>[15x]SM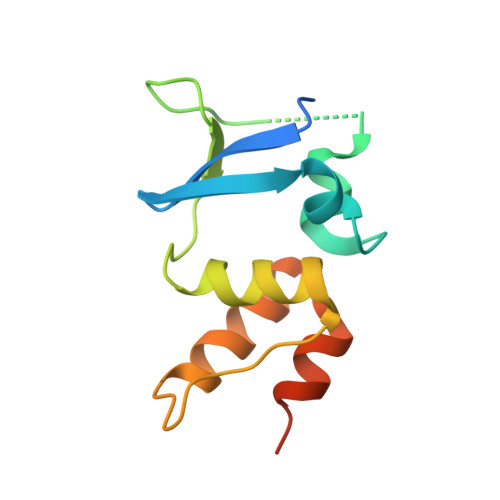GSAVPNSFPEVVELNVGGQVYFTRHSTLISIPHSLLWKMFSPKRDTANDLAKDSKGRFFIDRDGFLFRYILDYLRDRQVVLPDHFPEKGRLKREAEYFQLPDLVKLLTPDEIKQSPDE> MRDSNNIKYVREDAKKMHKLWAHIRMAMEGSRAIKDNAKEFVPHPDNTKATTPEGVARYKAYIERAVWYGASANTVDGMLGQIFARDPVFTGPEDKFDMLINDVDGSGLSIHQQARDSAEDALSLGRGGLFVDYSYVTTNGVSEAQEESGEARPYIKFIAAEDILNWRERWVNGAKRTTLLVF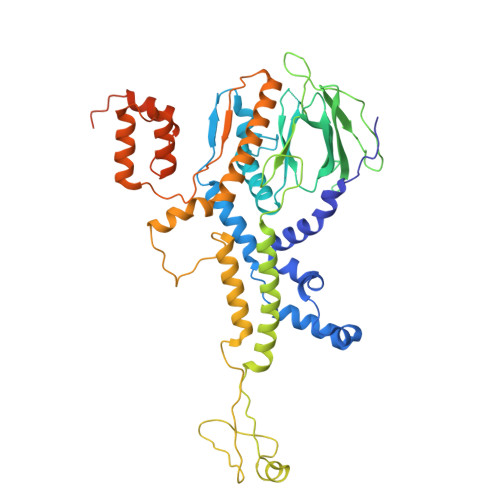REESDADDDGYQIYKEEVWRELRLVDGTYWQRTWRENDGQLYVDDWISPTKADGSQFDEIPFVIFGSKNNDPTIDMPPMRDLVELNIAHFRNSADYEEACFICGQPTLFLSGLTEHWVKNVLGGAVVIGSRDAVPLPVNAKPELLQAEGNGMVKEAMDQKERQMVALGAKLIDSDKTQRTFGEASMEAAAQNSVLSRVSKNVSDAYTKALRWAAMFLGLDEKIEYELNSDFDINKMSPEELAAVISAWQSNAISFTEMRWQIKKGGRAYLEDEDMRNESEQDDPLKLDITKPDPNEDPNASEDDQTDPNDETKEKDAETGGAE> GNRTFSY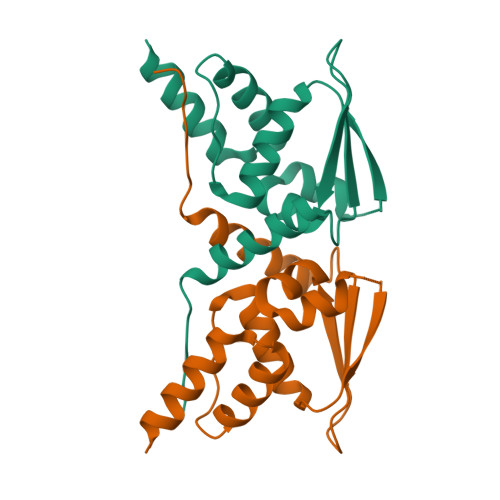TLEDHTKQAFGIMNELRLSQQLCDVTLQVKYQDAPAAQFMAHKVVLASSSPVFKAMFTNGLREQGMEVVSIEGIHPKVMERLIEFAYTASISMGEKCVLHVMNGAVMYQIDSVVRACADFLVQQLD> SY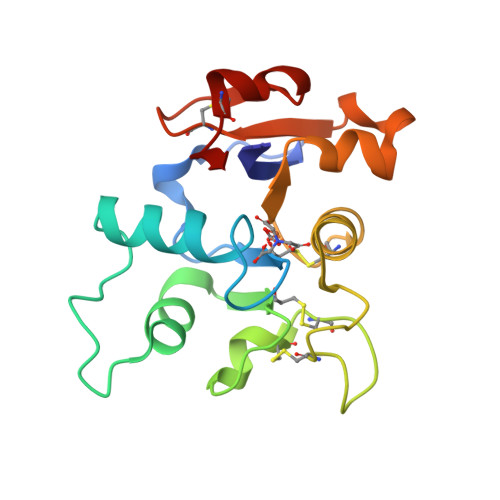YAVAVVKKGTDFMIKDLRGKTSCHTGLGRSAGWNIPIGTLIHRGDIEWEGIESGSVEQAVAKFFSASCVPGATTEQKLCRQCKGDAKTKCLRNAPYSGYSGAFQCLKDGKGDVAFVKHTTVQENAPEEKDEYELLCLDGTRQPVDSYKTCNWARV(8R)-3-(5-S-methyl-5-thio-beta-D-ribofuranosyl)-3,6,7,8-tetrahydroimidazo[4,5-d][1,3]diazepin-8-ol 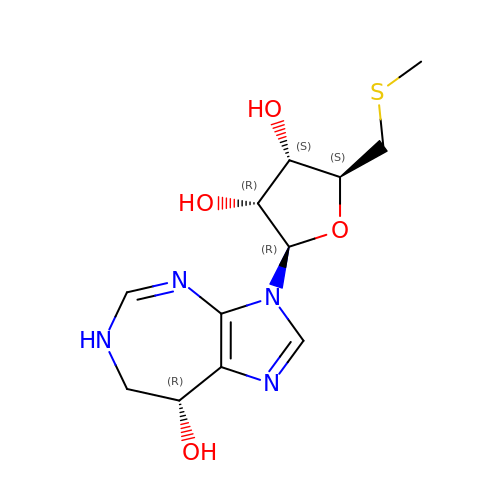| C12 H18 N4 O4 S | QLPPCUVJNCMYFD-SANHVUMCSA-N>ATFPKAMDNVTVRQGESATLRCTIDDRVTRVAWLNRSTILYAGNDKWSIDPRVIILVNTPTQYSIMIQNVDVYDEGPYTCSVQTDNHPKTSRVHLIVQVPPQIMNISSDITVNEGSSVTLLCLAIGRPEPTVTWRHLSVKEGQGFVSEDEYLEISDIKRDQSGEYECSALNDVAAPDVRKVKITVNYPPYISKAKNTGVSVGQKGILSCEASAVPMAEFQWFKEETRLATGLDGMRIENKGRMSTLTFFNVS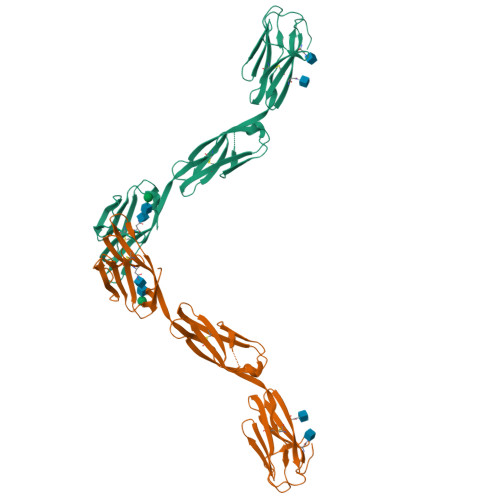EKDYGNYTCVATNKLGNTNASITLYGPGAALVPR[2x]> MSAQVMLEDMARKYAILAVKADKEGKVDDAITYYKKAIEVLSQIIVLYPESVARTA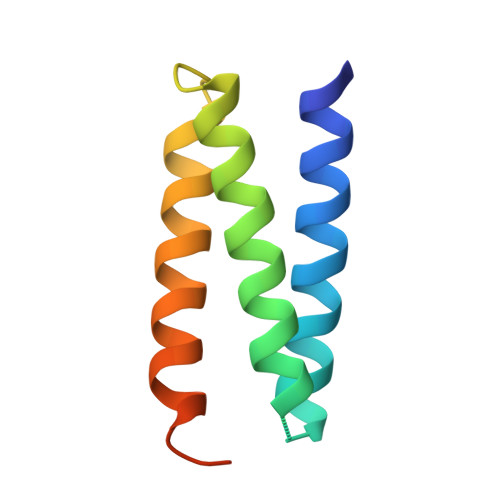YEQMINEYKKRISYLEKVLPASSDGSG>SNARAEFVNPFLASLMNVLKTMASLELKPQKPRIKKDEIARGDVSGLIGMVGAQTRGSMSITFDEGLALEIMQNMLGERPNGLNEEVTDMVGEITNMVTGGAKRILAESGFDFDMATPVVVSGKGHTI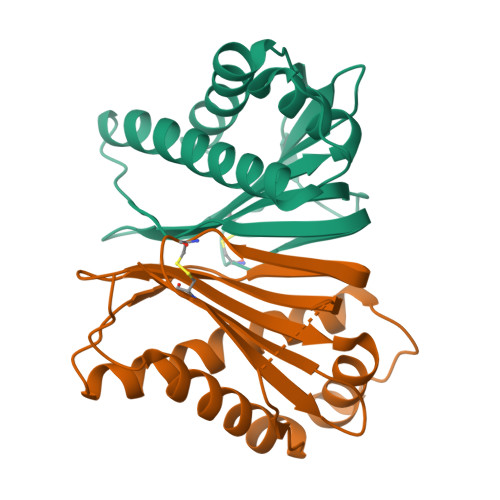RHKCEGSIIIMPFSSQWGNAFIEICFE[2x]> AREPLTSYLDSQYFGKIYIGTPPQEFTVVFDTGSSDLWVPSIYCKSNVCKNHHRFDPRKSSTFRNLGKPLSIHYGTGSMEGFLGYDTVTVSNIVDPNQTVGLSTEQPGEVFTYSEFDGILGLAYPSLASEYSVPVFDNMMDRHLVARDLFSVYMDRNGQGSMLTLGAIDPSYYTGSLHWVPVTLQQYWQFTVDSVTINGVAVACVGGCQAILDTGTSVLFGPSSDILKIQMAIGATENRYGEFDVNCGNLRSMPTVVFEINGRDYPLSPSAYTSKDQGFCTSGFQGDNNSELWILGDVFIREYYSVFDRANNRVGLAKAI

Bovine and camel chymosin are aspartic peptidases that are used industrially in cheese production. They cleave the Phe105-Met106 bond of the milk protein κ-casein, releasing its predominantly negatively charged C-terminus, which leads to the separation of the milk into curds and whey. Despite having 85% sequence identity, camel chymosin shows a 70% higher milk-clotting activity than bovine chymosin towards bovine milk. The substrate-binding cleft and active site are located at the interface of the two domains.

The doubly glycosylated variant 2 was used for the crystallization of camel chymosin. The crystals obtained by crystallization of variant 2 contained a protein lacking the first three residues of the N-terminus. The structural model of camel chymosin contains an NAG residue covalently bound to Asn100 and this does not appear to influence the atomic displacement parameters, which are similar to the values for bovine chymosin. The higher mobility of the loop containing Asn291 could explain why it was not possible to identify any carbohydrate bound to Asn291 in the electron density, even though mass spectrometry of the crystals had shown that camel chymosin was glycosylated at both sites. The first ten residues are not visible in camel chymosin. The disordered N-terminus of camel chymosin implies that this structure lacks one of the strands, which leads to a breakdown of the pseudo-twofold symmetry that relates the two domains of the chymosin structure. The presence of the large charged Arg5 and Glu6 residues (Ser5 and Val6 in bovine chymosin) adjacent to each other precludes the participation of the N-terminus in the β-­sheet, as one of them must be buried in the hydrophobic core of the protein. In camel chymosin it blocks a major part of the binding cleft and must undergo a conformational change upon binding of substrate. The lack of hydrogen-bond partners for the β-strand formed by residues Leu166–Leu168 is compensated in camel chymosin by a slight displacement of the loop formed by residues 93–96, which enables the side chain of Ser94 to form a hydrogen bond to the carbonyl group of Leu166, thus connecting the β-strand to the loop 93–96. In addition, camel chymosin possesses a small positive patch on the C-terminal domain comprised of residues Arg242, Arg254 and Lys278 (part of the second patch); the corresponding residues in the bovine enzyme are hydrophilic but neutral.Contactins (CNTNs) are neural cell adhesion molecules that encode axon-target specificity during the patterning of the vertebrate visual and olfactory systems. Because CNTNs are tethered to the plasma membrane by a glycosylphosphatidylinositol anchor, they lack an intracellular region to communicate across the membrane. Instead, they form coreceptor complexes with distinct transmembrane proteins to transmit signals inside the cell. Finally, structural analyses of five CNTN–amyloid pairs indicate that these proteins interact through a conserved interface involving the second fibronectin type III repeat of CNTNs and the copper-binding domain of amyloid proteins.

We thus initiated crystallization trials with the E1 domain of mouse APP and the FN1–FN3 regions of mouse CNTN3 and CNTN5 but only succeeded in obtaining a crystal structure of the CNTN5–APP complex at moderate resolution (3.5 Å, Rwork/Rfree = 0.243/0.291). Overall, the binding sites identified in the structures of the CNTN5–APP complex and the CNTN3–APP fusion protein are similar to the one identified in CNTN4–APP structure. Residue H137 in APP contacts Y681 in CNTN3 (Y853 in CNTN5), and its side chain forms a hydrogen bond with the carboxylate group of E686 (D858 in CNTN5). Finally, even though residues T751 and V752 in chicken CNTN4 are replaced by K823 and M824 in mouse CNTN5, these lysine and arginine residues still form a hydrogen bond with S124 and van der Waals interactions with H137, respectively. We found it interesting that larger residues such as lysine and methionine would mediate interactions identical to threonine and valine and wondered whether these changes would shift the respective positions of CNTN5 and APP, thus affecting the “fit” in the complex. Indeed, the shape complementarity coefficient SC for CNTN4–APP is 0.78, whereas it is only 0.65 for CNTN5–APP. In CNTN5, the arrangement of residues surrounding APP A126 is distinct because the Cξ atom of F833 is located 5.3 Å away from the Cβ of A126, which is too far to mediate a van der Waals interaction. In this complex, A126 only contacts the aliphatic portion of K821 and the side chain of Y835, which, respectively, replace the methionine and phenylalanine residues that abut A126 in the CNTN4–APP and CNTN4–APPb complexes.

>GSTGSPPGPPGVVIVEEITESTATLSWSPATDNHSPISSYNLQARSPFSLGWQTVKTVPEVITGDMESAMAVDLNPWVEYEFRVVATNPIGTGDPSIPSRMIRTNEAVPKTAPSNVSGRSGRRHELVIAWEPVSEEFQNGEGFGYIVAFRPNGTRGWKEKMVTSSEASKFIYRDESVPPLTPFEVKVGVYNNKGDGPFSQIVVICSAEGEPTAAPTDVTATSVSVSEIFVVWKHVKESLGRPQGFEISYWKDTEPEDSVETVRTRGNESFVMLTGLEGNTLYHLTVRAYNGAGYGPPSREASTTTKR[2x];>GPGSEVPTDGNAGLLAEPQIAMFCGKLNMHMNVQNGKWESDPSGTKTCIGTKEGILQYCQEVYPELQITNVVEANQPVTIQNWCKRGRKQCKTHTHIVIPYRCLVGEFVSDALLVPDKCKFLHQERMDVCETHLHWHTVAKETCSEKSTNLHDYGMLLPCGIDKFRGVEFVCCPLA[2x]>MSKVPVVGIVAALLPEMGIGFQGNLPWRLAKEMKYFREV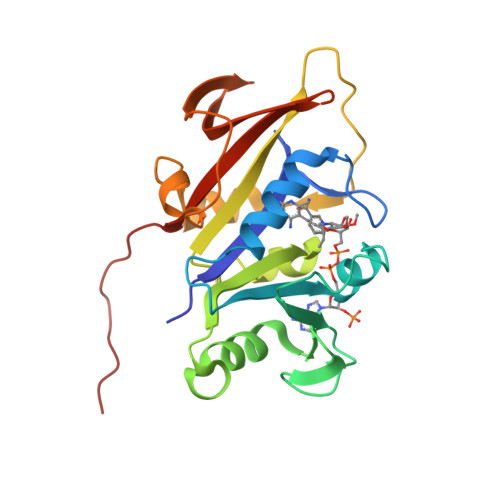TTLTNDNSKQNVVIMGRKTWESIPQKFRPLPKRINVVVSRSFDGELRKVEDGIYHSNSLRNCLTALQSSLANENKIERIYIIGGGEIYRQSMDLADHWLITKIMPLPETTIPQMDTFLQKQELEQRFYDNSDKLVDFLPSSIQLEGRLTSQEWNGELVKGLPVQEKGYQFYFTLYTKKLEHHHHHHHH[2x]> GLSRGPSPISLSAQESWPVAAAITEYINAYFRGGEHNRCLVKITGDLTMSFPAGITRIFTANPNAPVLSFRLVNISRVDHFLPNQKL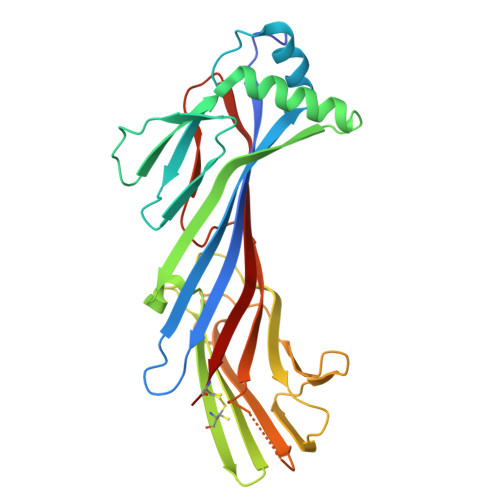LYSDPSQSDPDTKDFWFNMQALTLHLQREAELNPQASYYNVALLKYQASSQDPSRAPLLLSAECQRSGTVTRVSLDYHCCPATAPATQLTSVQVLLPLDHSATDLQCQPPAAWNAEERRLLWKLANLSPTNHSKGSGTLCASWQCLEVPRGPAPSLAVQFVGSGASLSGLDVELVGSRYRMSLVKKRFATGKYMAGCSL In bacteria, topoisomerase IV, a tetramer of two ParC and two ParE subunits, unlinks daughter chromosomes prior to cell division, whereas the related enzyme gyrase, a GyrA2GyrB2 tetramer, supercoils DNA and helps unwind DNA at replication forks. Both enzymes act via a double-strand DNA break involving a cleavage complex and are targets for quinolone antimicrobials that act by trapping these enzymes at the DNA-cleavage stage and preventing strand re-joining. Levofloxacin is a broad-spectrum third-generation fluoro­quinolone antibiotic. It is active against Gram-positive and Gram-negative bacteria and functions by inhibiting gyrase and topoisomerase IV.

The crystallized complex was formed by turning over the topoisomerase tetramer in the presence of DNA and levofloxacin and crystallizing the product. In both cases the DNA is bent into a U-form and bound snugly against the protein of the G-gate. The methylpiperazine at C7 (using the conventional quinolone numbering; C9 in the IUPAC numbering) on the drug extends towards residues Glu474 and Glu475 for S. pneumoniae and towards Gln460 and Glu461 for K. pneumoniae, where the glutamate at 474 is substituted by a glutamine at 460 in the Klebsiella strain. For S. pneumoniae topoisomerase IV, one of the O atoms of the carboxyl of Asp83 points towards the Mg2+ ion and is within hydrogen-bonding distance (5.04 Å) through an Mg2+-coordinated water. Similar behaviour was observed for the S. pneumoniae topo­isomerase IV ParE30-ParC55 fusion protein. The CC25 (the drug concentration that converted 25% of the supercoiled DNA substrate to a linear form) was 0.5 µM for the Klebsiella enzyme and 1 µM for the pneumococcal enzyme.

>MSNIQNMSLEDIMGERFGRYSKYIIQDRALPDIRDGLKPVQRRILYSMNKDSNTFDKSYRKSAKSVGNIMGNFHPHGDSSIYDAMVRMSQNWKNREILVEMHGNNGSMDGDPPAAMRYTEARLSEIAGYLLQDIEKKTVPFAWNFDDTEKEPTVLPAAFPNLLVNGSTGISAGYATDIPPHNLAEVIDAAVYMIDHPTAKIDKLMEFLPGPDFPTGAIIQGRDEIKKAYETGKGRVVVRSKTEIEKLKGGKEQIVITEIPYEINKANLVKKIDDVRVNNKVAGIAEVRDESDRDGLRIAIELKKDANTELVLNYLFKYTDLQINYNFNMVAIDNFTPRQVGIVPILSSYIAHRREVILARSRFDKEKAEKRLHIVEGLIRVISILDEVIALIRASENKADAKENLKVSYDFTEEQAEAIVTLQLYRLTNTDVVVLQEEEAELREKIAMLAAIIGDERTMYNLMKKELREVKKKFATPRLSSLEDTAKALEHHHHHH[2x];>[2x]MGHHHHHHHHHHSSGHIDDDDKHMKNKKDKGLLSGKLTPAQSKNPAKNELYLVEGDSAGGSAKQGRDRKFQAILPLRGKVINTAKAKMADILKNEEINTMIYTIGAGVGADFSIEDANYDKIIIMTDADTDGAHIQTLLLTFFYRYMRPLVEAGHVYIALPPLYKMSKGKGKKEEVAYAWTDGELEELRKQFGKGATLQRYKGLGEMNADQLWETTMNPETRTLIRVTIEDLARAERRVNVLMGDKVEPRRKWIEDNVKFTLEEATVF> X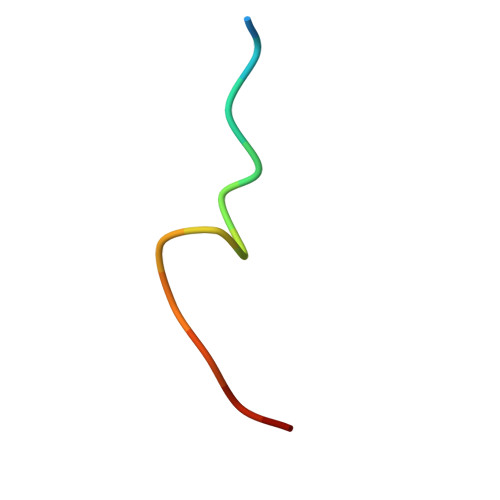RQCSMTCFYHSKX> MGSSHHHHHHSSENLYFQGHMATESPATRRVQVAEHPRLLKLKEMFNSKFGSIPKFYVRAPGRVNIIGEHIDYCGYSVLPMAVEQDVLIAVEPVKTYALQLANTNPLYPDFSTSANNIQIDKTKPLWHNYFLCGLKGIQEHFGLSNLTGMNCLVDGNIPPSSGLSSSSALVCCAGLVTLTVLGRNLSKVELAEICAKSERYIGT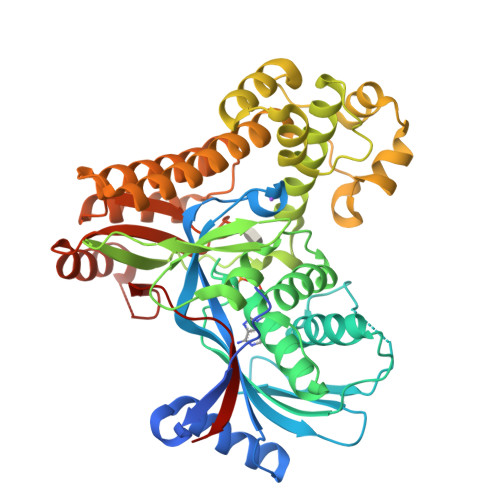EGGGMDQSISFLAEEGTAKLIEFSPLRATDVKLPSGAVFVIANSCVEMNKAATSHFNIRVMECRLAAKLLAKYKSLQWDKVLRLEEVQAKLGISLEEMLLVTEDALHPEPYNPEEICRCLGISLEELRTQILSPNTQDVLIFKLYQRAKHVYSEAARVLQFKKICEEAPENMVQLLGELMNQSHMSCRDMYECSCPELDQLVDICRKFGAQGSRLTGAGWGGCTVSMVPADKLPSFLANVHKAYYQRSDGSLAPEKQSLFATKPGGGALVLLEA>[4x]AFAKIEEGKLVIHMPAAVAVTSPQADSAPAQRFSLPQGCHFRTFWRDEANGGSLFIPAGDALRCGEDGWLQGSGAVTLQQGGQTLSPT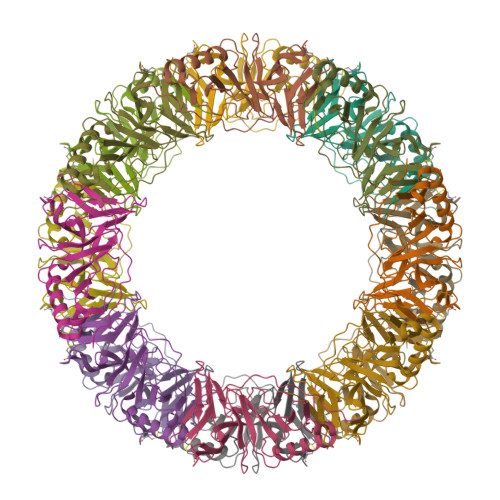LWFLQGYPLAQVNGGDRALTVVSANAQRLILGGNPQAPGSFLLLTFEPQLHAWAFNGEAIVEMPRVDAADETKIKQRVQQAQTAWQPLLSAPAPLTFKLVEKLAADRVDPASGSYLSVNGATHLEGSEFKLVDHHHHHH>GHMMSVNEEQFGSLYSDERDKPLLSPTAQKKFEEYQNKLANLSKIIRENEGNEVSPWQEWENGLRQIYKEMIYDAFDALGVEMPKDMEVHFAGSLAKAQATEYSDLDAFVIVKNDEDIKKVKPVFDALNNLCQRIFTAS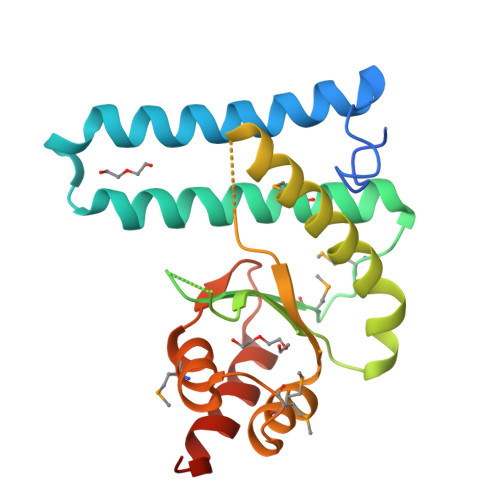NQIYPDPIGINPSRLIGTPDDLFGMLKDGMVADVEATAMSILTSKPVLPRYELGEELRDKIKQEPSFSNMVSAK[2x]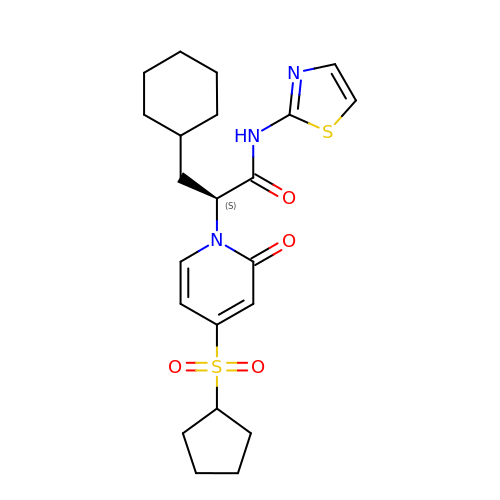(2S)-3-cyclohexyl-2-[4-(cyclopentylsulfonyl)-2-oxopyridin-1(2H)-yl]-N-(1,3-thiazol-2-yl)propanamide | C22 H29 N3 O4 S2 | AIIAMUOQMJYEJH-IBGZPJMESA-N> SMTTRPAESAPQTASTLLEPGSNGVVRLLGGPGTGKSSLLVDTAVQHILAGADPESVLLLTGSARLRTAARAAITARLLGAGTVGVVREPLVRTVHSYAFAVLRLAAQRNGDPPPRLITSAEQDGIIRELLAGDLEDGHRSPVGWPEQLWPALTTAGFATELRDLMARCTERGVDPIALQRLGRTAKRPEWLAAGRFAQAYEQIMLLRSAVGMAAPQATVPALGAAELVGAALEALGADDELLDTERNRIKLLLVDDAQHLDPQAARLVRALAAGTGLTVIAGDPDQSVFGYRGADPVLLRDDTHPAITLTQSYRCAPEIASAITGLGQRLPGVSDTRHWTGNPQREGTVTVRLAASTHAEGTMIADALRRAHLVDGIPWSQMAVIVRSVPRVGTALARALTAAGVPVQDNGTDVPVGRQPAAAALLTVLDVTATGHLDADSAVALLTGPIGRVDPVTLRQLRRALRRADGSQPPRDFGDLLVDAIEREPKGLSAEHARTLRRLRAVLTAARRSDASGADPRYTLWQAWHASGLQRRWLAASERGGSVGAQADRDLDAVTTLFDVADQYVNRTAGASLRGLVDHVTRLGAAVARTEPETAAEAVAVLSVHGALAGEWDFVVIAGVQEGLWPNMIPRGGVLGTQHLVDVLDGVADMTDRTVSTRAPLVAEERRLLMAAMGRARTRVMITAVDSDTGDESLLPSPFCAEISAWATEPVAEPPLVAPRVLAPSALVGRLRAVVCAPDGAVDDDARACAAAQLARLAAAGVPGADPSQWHAMTSLTTEEPLWSEPGHVVTLSPSTLQMLTDCPLRWLLERHGGDDGRDVRSTVGSLVHALVSEPGKTESQLVNELEKVWDDLPYDAKWYSDNELARHRAMLETFTRWREDTRRQLTEVATEIPVEGIVVEPGENTPGVRVRGRLDRLERDEAGRLVVVDLKTGKSPVTKDDAQNHAQLAMYQLAVAAGLLDDGDEPGGGKLVYLGKAGAAGATEREQDPLTPDKRAEWLETVGEAAAATAGPRFVARVNNGCANCPVRSSCPAQANGDRP;> MTQVASPVVQARYSPVELSAALGLFPPTDEQAAVIAAPPGPLVVIAGAGAGKTETMAARVVWLVANGFATPSQVLGLTFTRKAAGQLLRRVRTRLARLAGAGLAPGSGASDESATVSTYHAFAGTLLREHGLLLPVEPDTRLLSETELWQLAYDVVCAHPGHLDTEKTPAAVTAMVLRLSGALAEHLVDTDQLRDTHVELERLVHTLPAGPYQRDRGPSQWLLRMLATQTERTELVPLIDALHQRMRAEKVMDFGMQMAAAARLAARFPQVGEQLRQRFRVVLLDEYQDTGHAQRIALSSLFGGGADDGLALTAVGDPIQSIYGARGASATNLPRFTTDFPYSDGTPAPTLELRTSWRN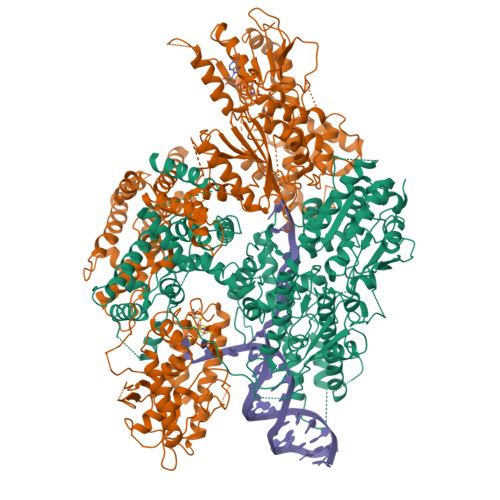PPSTLHVANAVSEEARRRSVAVRALRPRPDAEPGTIRCALLNNVAAERDWVADHLARAYHGAIGRGEAAPTAAVLVRRNADAAPMAEALTARGVPVEVVGVAGLLAVPEVADLVAMLRLIADPTAGSAVMRILTGPRWRFGARDIAALWRRAVELDDRPKGELGTADIVAQAAPDADTACVADAICDPGDAERYSPAGYERIVALGRELTMLRAHLGHPLPELVAEVRRVLGLDAEARAARPVAAGWAGTENLDRFSDLVSDFAGHAGASVSALLAYLDAAVEVENGLAPAELTVSHDRVQILTVHAAKGLEWQVVAVPHLSARVFPSTTQARTWLTDASDLPPLLRGDRATESEIGVPVLDTSDIYDRKILSDKISDHKKSLDQRRVDEERRLLYVAITRAEDTLLLSGHHWGATESKPRGPSEFLCELKTILEEATAAGTPCGEIEHWAPDPAPGETNPLRDQVVEALWPPVASADDHVHRGAQLVAAAMAGEVSAEADQEGWAADVDALLAERERPPQQEDTELPGQLSVSTLVELSRDPKAALTRLRRRLPQRPDPHALLGTTFHEWVQRYFHAERLFDLDDLPGAVDSDSGRAVEESLAELQDAFVKSPWAARTPVEVEVPFDMVLGETVVRGRIDAVFAEPDGTTMVLDWKTGDPPETPEAKEHAAVQLAVYRLAWAAMRGCPPESVRAAFHYVRSGQTVIPETLPGAEELVKLLAAAPTETAEEADRIT[6-(benzyloxy)-1-benzofuran-3-yl]acetic acid | C17 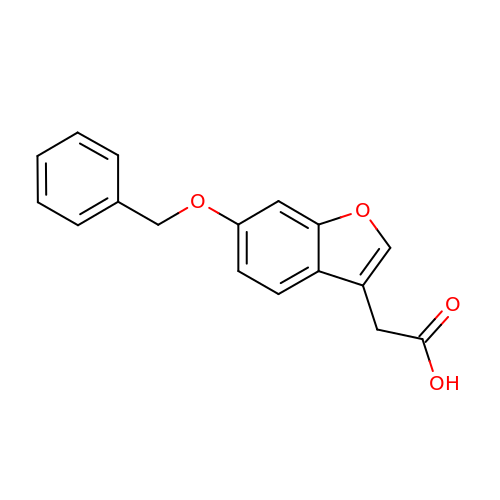H14 O4 | VJEZHKLENQLLAZ-UHFFFAOYSA-N4-[3-amino-6-(3,4,5-trimethoxyphenyl)pyrazin-2-yl]-2-methoxybenzoic acid | C21 H21 N3 O6 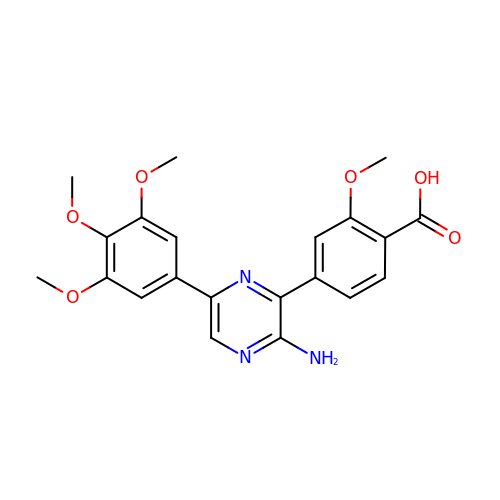| QYMUPWSODGEMOO-UHFFFAOYSA-N7-[5-(4-AMINO-5-HYDROXY-6-METHYL-TETRAHYDRO-PYRAN-2-YLOXY)-4-HYDROXY-6-METHYL-TETRAHYDRO-PYRAN-2-YLOXY]-6,9,11-TRIHYDROXY-9-(2-HYDROXY-ACETYL)-7,8,9,10-TETRAHYDRO-NAPHTHACENE-5,12-DIONE 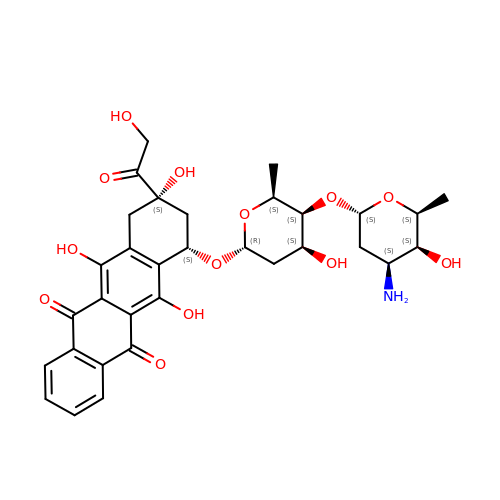| C32 H37 N O13 | VQHRZZISQVWPLK-UIRGBLDSSA-N>MISDSMTVEEIRLHLGLALKEKDFVVDKTGVKTIEIIGASFVADEPFIFGALNDEYIQRELEWYKSKSLFVKDIPGETPKIWQQVASSKGEINSNYGWAIWSEDNYAQYDMCLAELGQNPDSRRGIMIYTRPSMQFDYNKDGMSDFMCTNTVQYLIRDKKINAVVNMRSNDVVFGFRNDYAWQKYVLDKLVSDLNAGDSTRQYKAGSIIWNV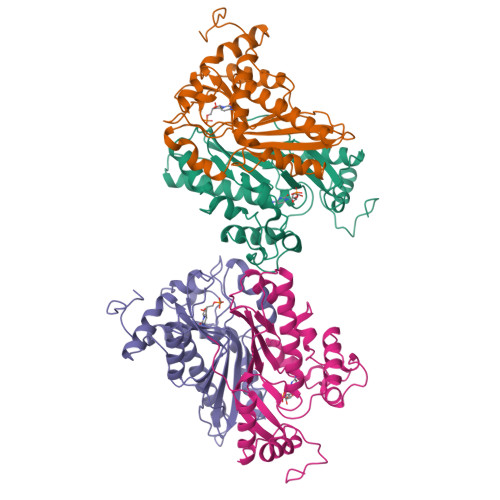GSLHVYSRHFYLVDHWWKTGETHISKKDYVGKYA[2x]> MGHHHHHHSSPKIEERTYPPQIPAQQELGDFSAYQSVLPEPLRKAEKLLQETGIKESTK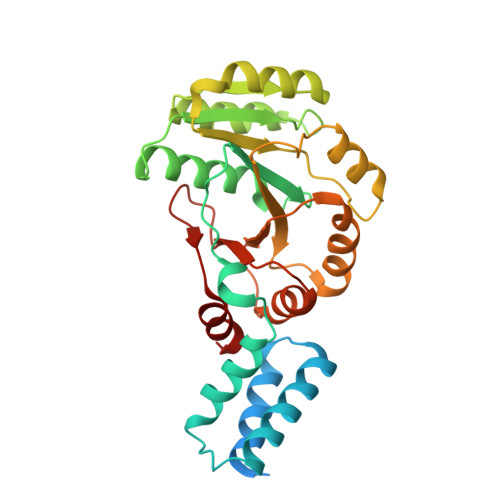TNTLKKLLRFSVEAGGLTEENVVGKLQEILCDMLPSADKWQEPIHSKYIVLFGSTGAGKTTTLAKLAAISMLEKHKKIAFITTDTYRIAAVEQLKTYAELLQAPLEVCYTKEEFQQAKELFSEYDHVFVDTAGRNFKDPQYIDELKETIPFESSIQSFLVLSATAKYEDMKHIVKRFSSVPVNQYIFTKIDETTSLGSVFNILAESKIGVGFMTNGQNVPEDIQTVSPLGFVRMLCR> MAP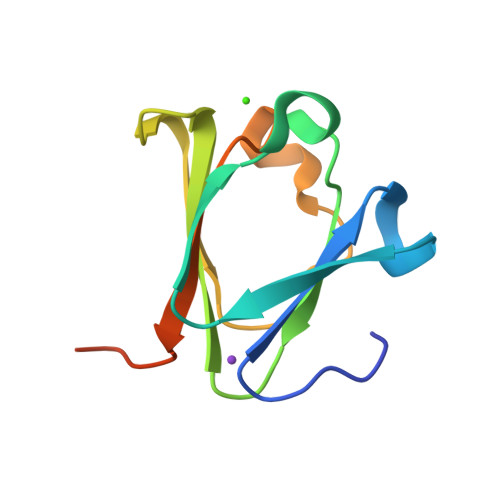SVDPTKVIFYQKKNFEGSGDTYAVGQDVSVPGSLNDKYFSVAVGASAKVIAWQHYNETGHYREWTTSQADISDIGGLSRFRVVDDDTRAISFLFKDAT> SQKVEKTVIKNETGTISISQLNKNVWVHTELGSFNGEAVPSNGLVLNTSKGLVLVDSSWDDKLTKELIEMVEKKFQKRVTDVIITHAHADRIGGIKTLKERGIKAHSTALTAELAKKNGYEEPLGDLQTVTNLKFGNMKVETFYPGKGHTEDNIVVWLPQYNILVGGSLVKST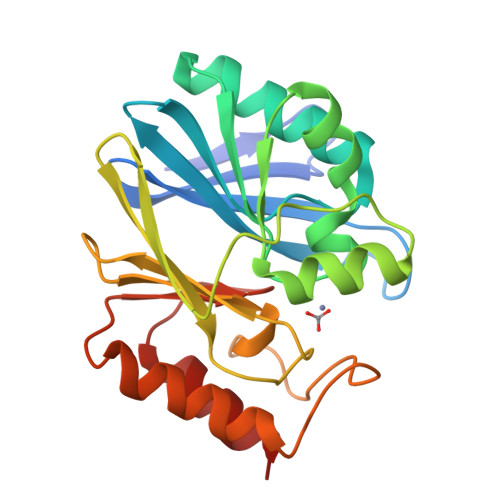SAKDLGNVADAYVNEWSTSIENVLKRYRNINAVVPGHGEVGDKGLLLHTLDLLK> MATLTDRSYFPPLGECLSGNKIILSWRLVATALEDLACDRLRSAAVSAFLRDGYVHQLLREPTKTFAPPTNETKLDFETKTGAINVVPSPNDPYNLDTIKDDARWLSRNVNINEVAALRVVIIEYQSRAHSHLTGPLSTQDVANVQEAAGVGDAQASAIVALLNVTTVADADSAWADFESETTRRRRLLATYLSERRSFLAAVDALLAFLLHSRAPGTGVELDPLRNAVLQGAFGFDQNAAKPDTTQLDALAPTYIRTLEGCFDRMQMAPESLDNQMLTEQFEVDWIRTALTEAIHAMSLIFQILDLKASQFAAPALVTQWFALMDTCEFFEPVPRGHELIAELLMPLHSLVAAISLKLLNVDRTLSYLDQDVDLLEEEEPYLASSDNLAQMHTTIAAAASAGLISTMPVVFAWSLILHQMHVGYQERAERRDLLQNQRAQAGFELEYEPSGRQRRNSAGSIVSIEASSYDVFLVSQQLERNIEPAENMARIATGRGQVYELMADMAVCLGSGQLAAFRPVLGARARLTFQDLLKRSAHYVGYQAEPVSCLLSILSGGSQYWDISAEAPSNEKSALDIYTRMLSDDTLNVQYASQSRNRFPYEFLPFASMCRILSAALVSDNESSELITGLLVKNPSLTLNWDPRWDRSYELVFEEENTNSFRLTKDIDLFDAASKSNRRILPEEKCTISRGTFGRFVTDVGRVAKLEFEHSTLALFGKRLEVNLMAGAYDTALGYLSADELIEGISLLATVLRAETLRSSKTDPDRGLRILTEASRLLSRGRDIMNVVCDTLDSLVEEELADLDGPKTAALSSCLQFLHAALPVCPGRVWAYMARCPLINTDTRSGRLSRITANLDMLAERYDLLLSAVKLFSSLVDSAKTSAVQRRSGISVNSRAKGEENPWIGASDKIVSRVTLSIAQTSVDVFENSATWRFPSEVDRSVMIRDVVGIMHKLMLYTH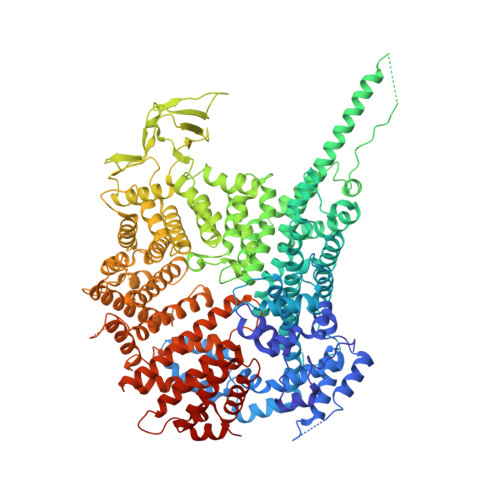SVGSTDTPRSLTGPLAPAADYVVESFLSSSSSSLRFQPLLATLLAAFQLPDTTIYQRRAQIVSERLTTVLEFATILLRVADYLNKASAGIQTQLFKSACVIARLPAIRHSFRIPAISLLSALVESAGKSSGEPPSLLGYLGPQVSRSFIQIAAQLDKPFDRVAEVASTWRFFSTILRNRQQWMANCLLTGKTPREALKGE6-azanyl-4-oxidanyl-naphthalene-2-sulfonic acid | C10 H9 N O4 S | 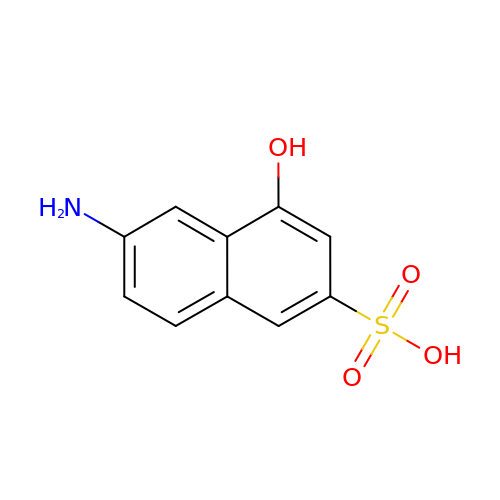HBZVNWNSRNTWPS-UHFFFAOYSA-N>GIRMTRISREMMKELLSVYFIMGSNNTKADPVTVVQKALKGGATLYQFREKGGDALTGEARIKFAEKAQAACREAGVPFIVNDDVELALNLKADGIHIGQEDANAKEVRAAIGDMILGVAAHTMSEVKQAEEDGADYVGLGPIYPTETKKDTRAVQ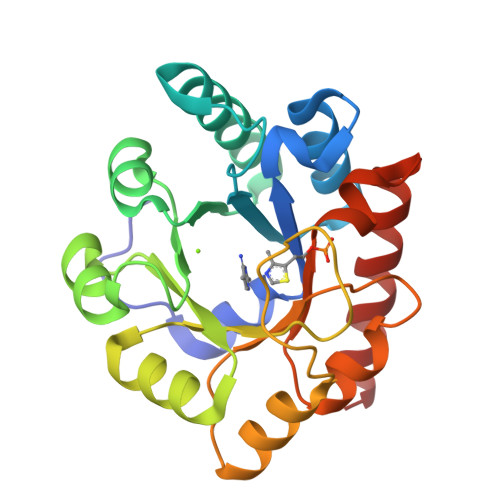GVSLIEAVRRQGISIPIVGIGGITIDNAAPVIQAGADGVSMISAISQAEDPESAARKFREEIQTYKTGR[2x]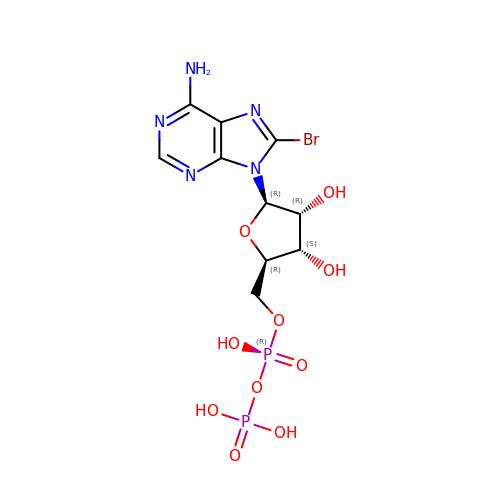8-BROMOADENOSINE-5'-DIPHOSPHATE | C10 H14 Br N5 O10 P2 | KVVVTFSHHQCHNZ-UUOKFMHZSA-N> MGSSHHHHHHSSGLVPRGSHSDEVDAHMSVASAVEVGVGEDEEEGVEEEEEEVEAVVMPERYALGGACRVLAGMPAPLGATALDGGVNFAVYSAGASAASLCLFTPDDLEADEVTE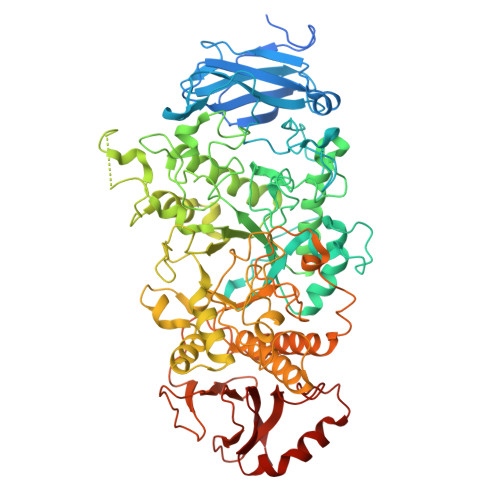EVPLDPLFNRTGNVWHVFIEGELHNMLYGYRFDGMFAPHCGQYFDVSNVVVDPYAKAVISRGEYGVPGPGGDCWPQMAGMIPLPYSTFDWQGDLPLRYPQKDLVIYEMHLRGFTKHSSSNVEHPGTYIGAISKLDYLKELGVNCVELMPCHEFNELEYFSCSSKMNFWGYSTINFFSPMIRYSSGGIRNCGRDAINEFKTFVREAHKRGIEVIMDVVFNHTAEGNEKGPILSFRGIDNSTYYMLAPKGEFYNYSGCGNTFNCNHPVVREFIVDCLRYWVTEMHVDGFRFDLASIMTRGCSLWDPVNVYGSPVEGDMTTTGTPLATPPLIDMISNDPILGDVKLIAEAWDAGGLYQVGQFPHWKIWSEWNGKYRDIVRQFIKGTDGFAGGFAECLCGSPHLYQAGGRKPWHSINFVCAHDGFTLADLVTYNKKYNSSNGEDNRDGENHNLSWNCGEEGEFAGLSVKRLRKRQMRNFFVSLMVSQGVPMFYMGDEYGHTKGGNNNTYCHDHYVNYFRWDKKEESSDLQRFCSLMTKFRKQCESLGLADFPTAQRLHWHGHQPGKPDWSETSRFVAFSTKDETKGEIYVAFNASHLPAVVGLPERPGYRWEPLVDTGKPAPYDFLTDDLPDRAHAVHLFSHFLNSNLYPMLSYSSIILELQPDD> MPVITVNTNVAEKSIPVFFQAALTNMMTKALQKPKEVMFVDLRSGANIMMGGDRNPCVFATVECIGRLNPTSNLAMARDMEDMFIEHLNVRRERIVIRFIPVPALFCSFNGALHDVSIERDEDIISQAIAEYLHHHHH;> MPVITVNTNVAEKSIPVFFQAALTNMMTKALQKPKEVMFVDLRSGANIMMGGDRNPCVFATVECIGRLNPTSNLAMARDMEDMFIEHLNVRRERIVIRFIPVPALFCSFNGALHDVSIERDEDIISQAIAEYLHHHAHH;> PVITVNTNVAEKSIPVFFQAALTNMMTKALQKPKEVMFVDLRSGANIMMGGDRNPCVFATVECIGRLNPTSNLAMARDMEDMFIEHLNVRRERIVIRFIPVPALFCSFNGALHDVSIERDEDIISQAI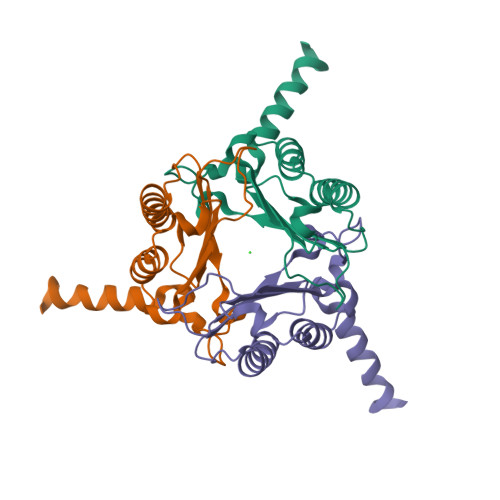AEYLHA;> MPVITVNTNVAEKSIPVFFQAALTNMMTKALQKPKEVMFVDLRSGANIMMGGDRNPCVFATVECIGRLNPTSNLAMARDMEDMFIEHLNVRRERIVIRFIPVPALFCSFNGALHDVSIERDEDIISQAIAEAAHHHA>MASWSHAPKFEKGASLDSPTFGCTDSPVRRERGQKAVFCGLTSIVWLHRKMQDAFFLVVGSRTCAHLLQAAAGVMIFAEPRFGTAVLEEQDLAGLADAHKELDREVAKLLERRPDIRQLFLVGSCPSEVLKLDLDRAAERLSGLHAPHVRVYSYTGSGLDTTFTQGEDTCLAAMVPTLDTTEAAELIVVGALPDVVEDQCLSLLTQLGVGPVRMLPARRSDIEPAVGPNTRFILAQPFLGETTGALERRGAKRIAAPFPFGEEGTTLWLKAVADAYGVSAEKFEAVTAAPRARAKKAIAAHLETLTGKSLFMFPDSQLEIPLARFLARECGMKTTEIATPFLHKAIMAPDLALLPSNTALTEGQDLEAQLDRHEAINPDLTVCGLGLANPLEAKGHATKWAIELVFTPVHFYEQAGDLAGLFSRPLRRRALLNGGAA[2x];>MKLTLWTYEGPPHVGAMRVATAMKDLQLVLHGPQGDTYADLLFTMIERRNARPPVSFSTFEASHMGTDTAILLKDALAAAHARYKPQAMAVALTCTAELLQDDPNGISRALNLPVPVVPLELPSYSRKENYGADETFRALVRALAVPMERTPEVTCNLLGATALGFRHRDDVAEVTKLLATMGIKVNVCAPLGASPDDLRKLGQAHFNVLMYPETGESAARHLERACKQPFTKIVPIGVGATRDFLAEVSKITGLPVVTDESTLRQPWWSASVDSTYLTGKRVFIFGDGTHVIAAARIAAKEVGFEVVGMGCYN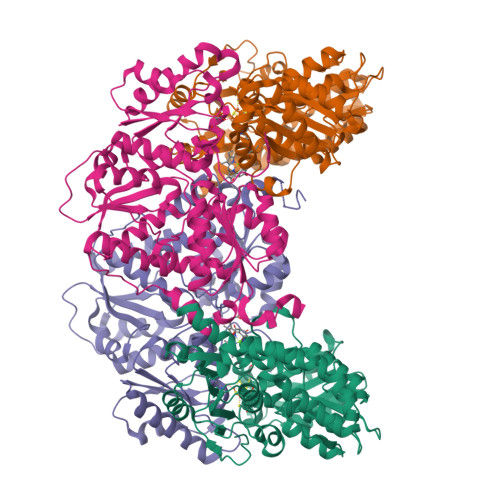REMARPLRTAAAEYGLEALITDDYLEVEKAIEAAAPELILGTQMERNIAKKLGLPCAVISAPVHVQDFPARYAPQMGFEGANVLFDTWVHPLVMGLEEHLLTMFREDFEFHDAAGASHHGGKAVAREESPVAPADLAPAATSDTPAAPSPVVVTQASGEIRWMPEAERELRKIPFFVRGKAKRNTELYAAHKGVCDITVETLYEAKAHYAR[2x]The surfaces of most bacteria and archaea are covered with a proteinaceous coat, the surface or S-layer, which is formed through the self-assembly of individual protein subunits into a regularly spaced, two-dimensional array. In C. difficile, the S-layer largely consists of a major S-layer protein, SlpA, which assembles into a paracrystalline array enveloping the cell. The major protein of the C. difficile S-layer, SlpA, is post-translationally cleaved into two S-layer proteins (SLPs): the high molecular weight (HMW) and low molecular weight (LMW), herein referred to as SLPH and SLPL, respectively. These subunits then form a complex (referred to as H/L) that is incorporated in the S-layer.

Conformational flexibility in the organisation of SlpA is further demonstrated by different arrangements observed in the structure of a truncated derivative of SlpA (SLPL/HID) and the H/L complex. Our models indicate the presence of a hinge, formed by the D1-LID linker. Analysis of the architecture and simulated motions (DynDom6D v1.0) in these models identified regions of D1-D2 and LID/HID as two dynamic domains, with the residues making up the linker between the D1 C-terminal β-strand (β17L) and the LID N-terminal β-strand (β18L) acting as an interdomain hinge. The calculated rotation angle of the centres of mass of the D1-D2 region relative to LID/HID of 166° suggests a high degree of flexibility of these regions, at least in the absence of the CWB2-containing SLPH core, with minimal effects on the fold of each individual domain. The fact that we observed this conformational flexibility in our protein crystal models, with no apparent effect on the fold of individual regions, suggests how the effector domains of other CWPs inserted in the functional S-layer can be accommodated by flexible rearrangement of D2. The strikingly different arrangements of the D1-D2 domains in SLPL, relative to the interacting domains observed in the H/L and SLPL/HID structures, are consistent with this proposed flexibility.

>MADSTTPGYTVVKNDWKKAVKQLQDGLKNKTISTIKVSFNGNSVGEVTPASSGAKKADRDAAAEKLYNLVNTQLDKLGDGDYVDFEVTYNLATQIITKAEAEAVLTKLQQYNDKVLINSATDTVKGMVSDTQVDSKNVAANPLKVSDMYTIPSAITGSDDSGYSIAKPTEKTTSLLYGTVGDATAGKAITVDTASNEAFAGNGKVIDYNKSFKATVQGDGTVKTSGVVLKDASDMAATGTIKVRVTSAKEESIDVDSSSYISAENLAKKYVFNPKEVSEAYNAIVALQNDGIESDLVQLVNGKYQVIFYPEGKRLETKS[2x];> MADIIADADSPAKITIKANKLKDLKDYVDDLKTYNNTYSNVVLEHHHHHH>MNMYSMPGYFQNMPTIGKELVNPNPENEQEIKAVESDIHESIKKALDAGITSEEKLNERGQLSAMQRINALIDPGTWCPLNSLFNPENNKFGTTNIVNGLGRVDGKWVYIVASDNKKMAGAWVPGQAENLIRCSDAAKMMHLPLIYLLNCSGVEFPNQDKVYPNRRGGGTPFFRNSELNQLGIPVIVGIYGTNPAGGGYHSISPTILIAHQDANMAVGGAGILSGMNPKGYIDDEAAEQIIAAQIENSKLKVPAPGSVPIHYDETGFFREVYQNDLGVIDGIKKYISYLPAYNLEFFRVDTPKAPQLPAEDLYSIIPMNQKRPYDIYEVIARLFDNSEFSEYKKGYGPEMVTGLAKVNGLLVGVIANVQGLLMNYPEYKQNSVGIGGKLYRQGLIKMNEFVTLCARDRIPLIWLQDTTGIDVGDEAEKAELLGLGQSLIYSIENSKLPSLEITIRKASAAAHYVLGGPQGNNTNVFSIGTGACEYYVMPGETAANAMYSRKLVKAKKAGEDLQPIIGKMNDMIQMYTDKSRPKYCTEKGMVDEIVDMTEVRPYIQAFTEAAYQNPQS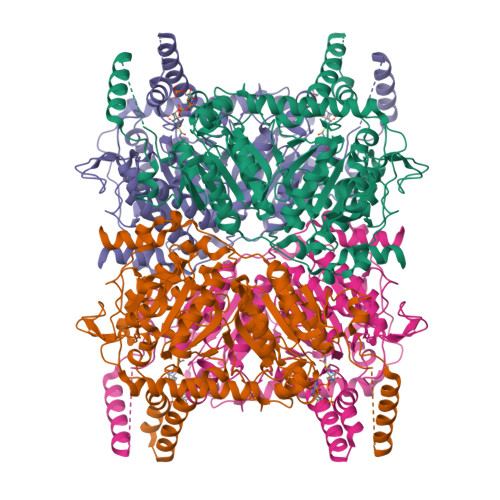ICPMHQMLTPRSTREFETFGK[2x]>PEIITPIITPFTKDNRIDKEKLKIHAENLIRKGIDKLFVNGTTGLGPSLSPEEKLENLKAVYDVTNKIIFQVGGLNLDDAIRLAKLSKDFDIVGIASYAPYYYPRMSEKHLVKYFKTLCEVSPHPVYLYNVPTATGKDIDAKVAKEIGCFTGVKDCIENIIHTLDYKRLNP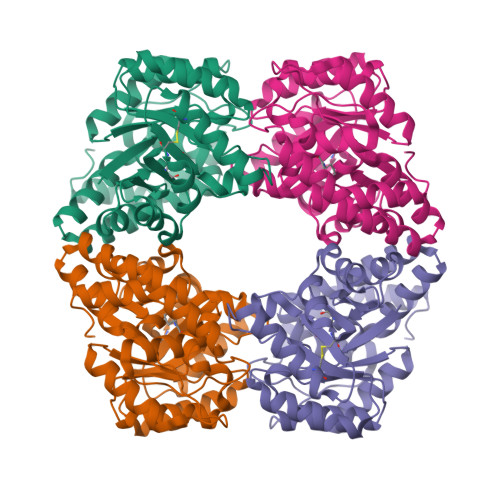NMLVYSGSDMLIATVASTGLDGNVAAGSNYLPEVTVTIKKLAMERKIDEALKLQFLHDEVIEASRIFGSLSSNYVLTKYFQGYDLGYPRPPIFPLDDEEERQLIKKVEGIRAKLVELKILKE[2x]> SNAMLNTLIVGASGYAGAELVTYVNRHPHMNITALTVSAQSNDAGKLISDLHPQLKGIVELPLQPMSDISEFSPGVDVVFLATAHEVSHDLAPQFLEAGCVVFDLSGAFRVNDATFYEKYYGFTHQYPELLEQAAYGLAEWCGNKLK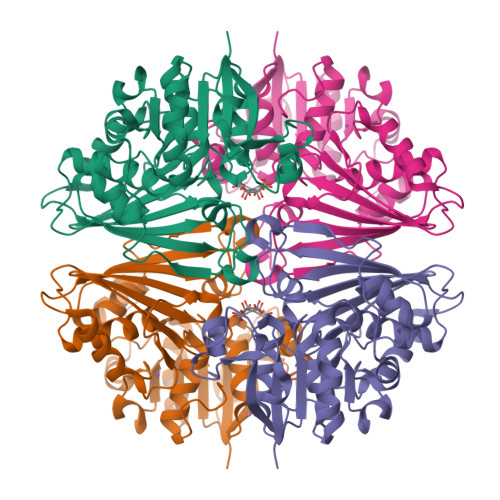EANLIAVPGCYPTAAQLALKPLIDADLLDLNQWPVINATSGVSGAGRKAAISNSFCEVSLQPYGVFTHRHQPEIATHLGADVIFTPHLGNFPRGILETITCRLKSGVTQAQVAQALQQAYAHKPLVRLYDKGVPALKNVVGLPFCDIGFAVQGEHLIIVATEDNLLKGAAAQAVQCANIRFGYAETQSLI>[2x]MGSSHHHHHHSSGLVPRGSMSDDTSLELPFTHRRNPHQTEAADRHLEWLQRHRELAAVVSGSTYTGWDITELASLVYPESSAEDLALAADLMGFYFLFDDQFDS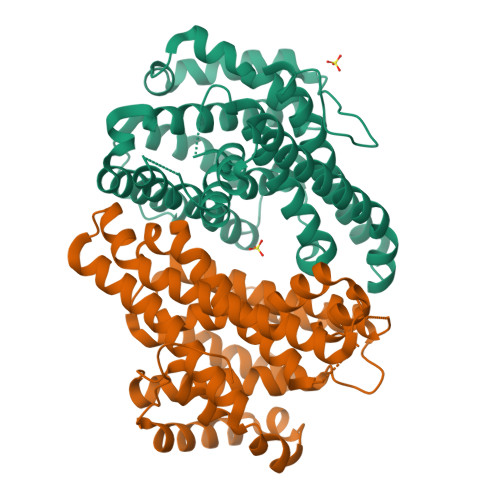PLGRRPEQVALICERLSAIAHGTLTAVTSPSERAFADLWRRITLGMTDRWRARAACNWEYYFACHPAEAAGRTIGQPPDREGYLTLRRGTAAMESIFDMIERLGHFEVPQHVMHHPLFRQLRQLAADIPSFTNDVRSFAQESERGDVANLVMIVRRDRCCSTAEACAVVWDEAQRMADRFCDLRDQLPDACRSMSLDPAQRLAAERYADGMALWLAGYLHWESHTRRYHHG>[5x]MKKLVMTAAVAAILGAASPVMAQGIPVFDGTRALDFVQQFARMKEQLDTAKDQLAEAQRMYEAVTGGRGLGDLMRNAQLR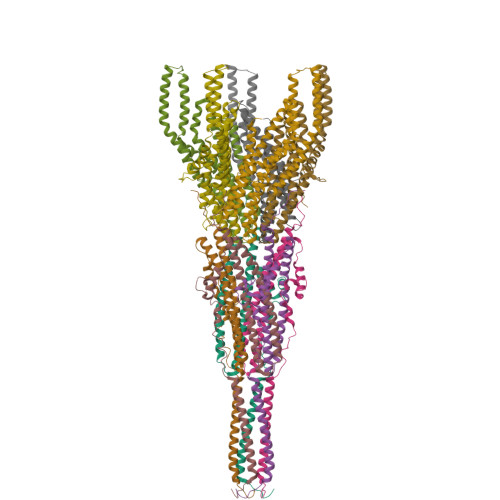EYLPDDLRTVYDSANGGGYSGISGSINDILRDERLNGSVADMRRSIEERSRTAAATDKAVGLRAYEGAQQRLAQIEGLMDEISRTQDQKAIEELQARIAGEQAAIQNETTKLQMIAQLRQAEQALISEQRRERNMRILSSGNQGMPTIQ;>MAFELFTPLFNKIDQTTATYVTDISSRAIAAITPVVSVGLTLGFITYGWLIIRGAVEMPVAEFLNRCLRIGIIVSIALAGGLYQGEIANAITTVPDELASALLGNPTQGASAAALVDQSAQQGFDRASEAFEEAGFFSSDGLLYGLFGIIILLATGLLAAIGGAFLLLAKIALALLAGLGPLFILALIWQPTHRFFDQWAQQVLNYGLLIVLFAAVFGLLMQIFGSYMADLRFDGAQNVAYAIGGSVILSIVSIVLLMQLPSIASGLAGGIGLGYMWELRSMRSGAGAAMRGGRAMARGARAAPGAARGAAVGAANMAKTVATGGAGVARAAAGYFRGRKAG[5x]>GSHMKPASFMTSICDERGQELIYAGMPITEVFKEEMGIGGVLGLLWFQKRLPKYSCQFIEMCLMVTADHGPAVSGAHNTIICARAGKDLVSSLTSGLLTIGDRFGGALDAAAKMFSKAFDSGIIPMEFVNKMKKEGKLIMGIGHRVKSINNPDMRVQILKDYVRQHFPATPLLDYALEVEKITTSKKPNLILNVDGLI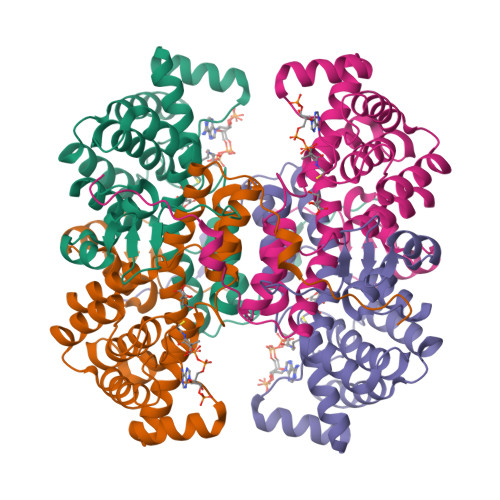GVAFVDMLRNCGSFTREEADEYIDIGALNGIFVLGRSMGFIGHYLDQKRLKQGLYRHPWDDISYVLPEHMSM[2x]>GFFSFIGEAFQGAGDMWRAYTDMKEAGWKDGDKYFHARGNYDAAQRGPGGVWAAEKISDAR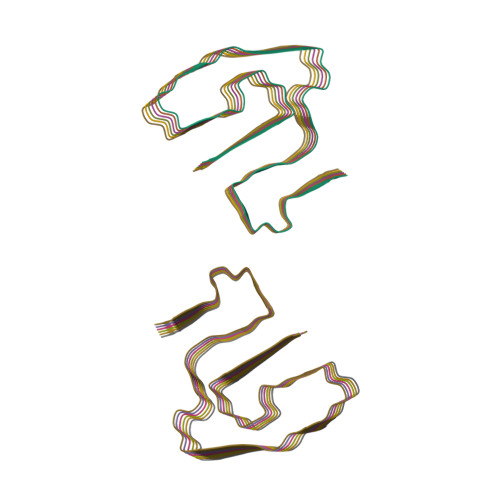ESFQEFFGRGHEDTMADQEANR[12x]> MSRKKMGLLVMAMGTPYKEEDIERYYTHIRRGRKPEPEMLQDLKDRYEAIGGISPLAQITEQQAHNLEQHLNEIQDEITFKAYIGLKHIEPFIEDAVAEMHKDGITEAVSIVLAPHFSTFSVQSYNKRAKEEAEKLGGLTITSVESWYDEPKFVTYWVDRVKETYASMPEDER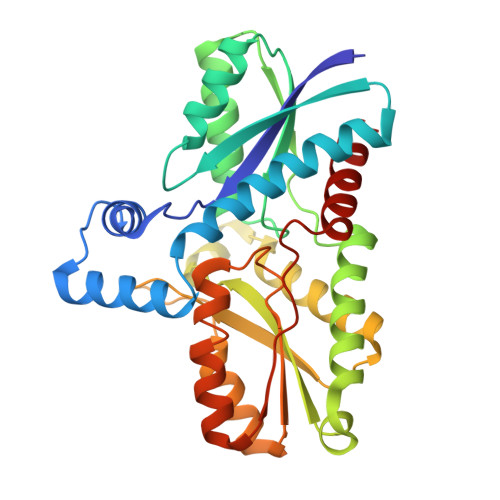ENAMLIVSAHSLPEKIKEFGDPYPDQLHESAKLIAEGAGVSEYAVGWQSEGNTPDPWLGPDVQDLTRDLFEQKGYQAFVYVPVGFVADHLEVLYDNDYECKVVTDDIGASYYRPEMPNAKPEFIDALATVVLKKLGR> MELCNILKYDRSLYPGKAVFFYKTADSDFVPLEADINKIRGPKSGFTEAFTPQFSPKNISPQDLTHNNILTLEECYVPPNVEHIFCRFSLRVQANSLVPSGCSDPEVFSLLKELAETFKECGGYKELAVRYCRNILIGTWLWRNQNTGNTQIEIKTSKGSCYLIDNTRKLAWESKWASDDLKVLEELSNEIESALTDPNVFWSADITAKIEASFCQEIYPSQILNDKVKQGEASKQFVKAKCADGRYAVSFNSVKIGAALQSIDDWWDEDASKRLRVHEFGADKEI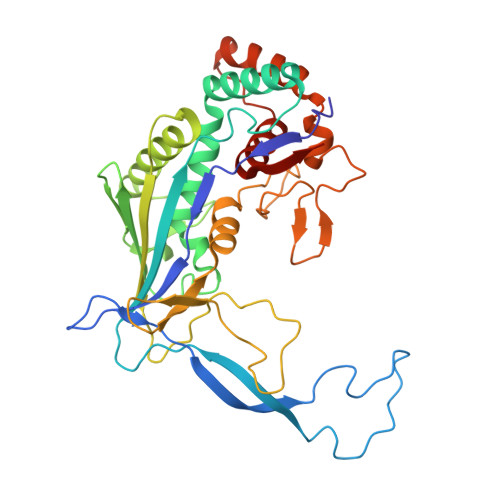GVARRPPDSEQNFYSIFKNTEWYLSALKNCITNKNEKIDPAIYYLFSVLIKGGMFQKKAEAKKA> PAAAPGKNFDLSHWKLQLPDANTTEISSANLGLGYTSQYFYTDTDGAMTFWAPTTGGTTANSSYPRSELREMLDPSNSKVNWGWQGTHTMKLSGKTVQLPSSGKIIVAQINGIMDDGTNAPPLVKAVFQDGQLDMQVKQNSDGTGSDVHNYFTGIKLGDLYNMEIRVTDGVAYVTMNGDT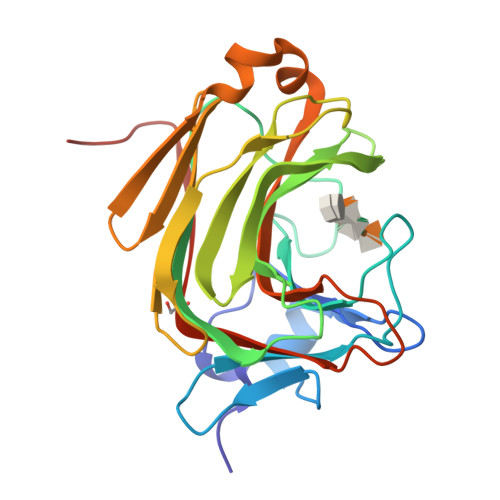RSVDFVGKDAGWKNLKYYFKAGNFVQDNTSTGGSAIAKLYSLSVSHSNLEHHHHHH> ALPQTVRIGTDTTAAPFSSKDAKGEFIGFDIDLGNEMCKRMQVKCTWVASDFDALIPSLKAKKIDAIISSLSITDKRQQEIAFSDKLYAADSRLIAAKGS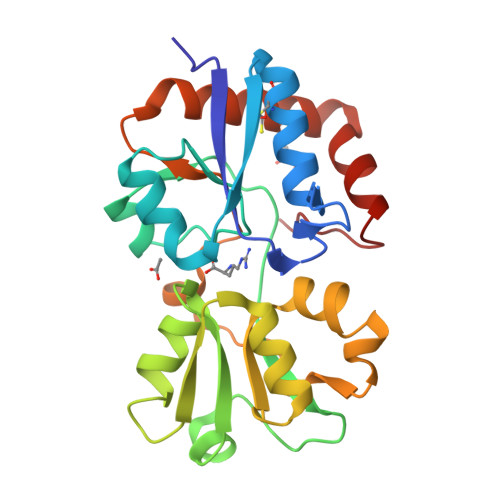PIQPTLESLKGKHVGVLQGSTQEAYANDNWRTKGVDVVAYANQDLIYSDLTAGRLDAALQDEVAASEGFLKQPAGKEYAFAGPSVKDKKYFGDGTGVGLRKDDTELKAAFDKALTELRQDGTYDKMAKKYFDFNVYGD>GMTVAAKSEIQIDNDEVRVTEWRLPPGSATGHHTHGMDYVVVPMADGEMTIVAPDGTRSLAQLKTGRSYARKAGVQHDVRNESTAEI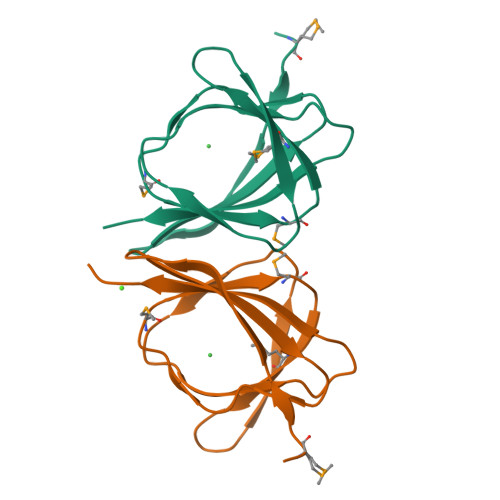VFLEIELKAGS[2x]>[2x]GSDESMEPSLPLTSVEPCVICQTRPKNGCIVHGRTGHLMAC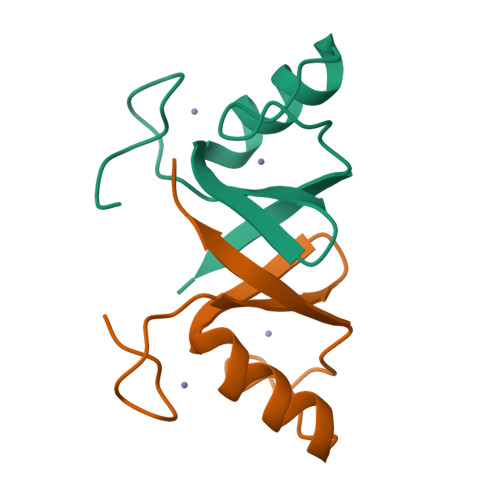YTCAKKLKKRNKPCPVCREPIQMIVLTYFS>[6x]GSEFGSGSNMSQWIRFRCSKIDEGGDWRPIVQFLRYQQIEFITFLGALKSFLKGTPKKNCLVFCGPANTGKSYFGMSFIHFIQGAVISFVNSTSHFWLEPLTDTKVAMLDDATTTCWTYFDTYMRNALDGNPISIDRKHKPLIQLKCPPILLTTNIHPAKDNRWPYLESRITVFEFPNAFPFDKNGNPVYEINDKNWKCFF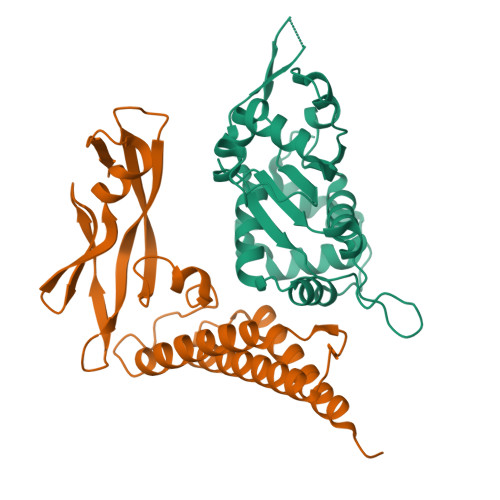ERTWSRLDLHE;>[6x]GSHMQTPKETLSERLSALQDKIIDHYENDSKDIDSQIQYWQLIRWENAIFFAAREHGIQTLNHQVVPAYNISKSKAHKAIELQMALQGLAQSAYKTEDWTLQDTCEELWNTEPTHCFKKGGQTVQVYFDGNKDNCMTYVAWDSVYYMTDAGTWDKTATCVSHRGLYYVKEGYNTFYIEFKSECEKYGNTGTWEVHFGNNVIDCNDSMCSTSDDTVSAT> MKLSKDTTALLKNFATINSGIMLKSGQFIMTRAVNGTTYAEANISDVIDFDVAIYDLNGFLGILSLVNDDAEISQSEDGNIKIADARSTIFWPAADPSTVVAPNKPIPFPVASAVTEIKAEDLQQLLRVSRGLQIDTIAITVKEGKIVINGFNKVED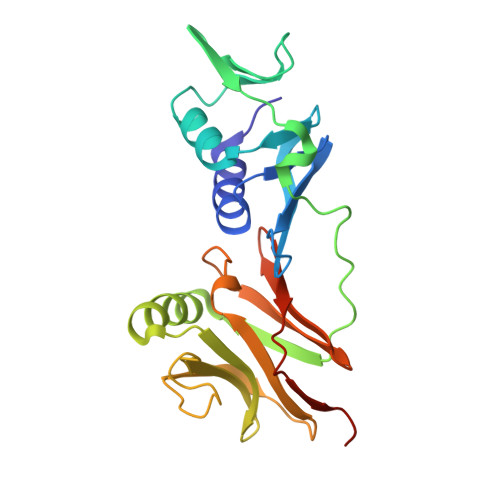SALTRVKYSLTLGDYDGENTFNFIINMANMKMQPGNYKLLLWAKGKQGAAKFEGEHANYVVALEADSTHDFLEHHHHHH>MASQPNSSAKKKEEKGKNIQVVVRCRPFNLAERKASAHSIVECDPVRKEVSVRTGGLADKSSRKTYTFDMVFGASTKQIDVYRSVVCPILDEVIMGYNCTIFAYGQTGTGKTFTMEGERSPNEEYTWEEDPLDGIIPRTLHQIFEKLTDNGTEFSVKVSLLEIYNEELFDLLNPSSDVSERLQMFDDPRNKRGVIIKGLEEITVHNKDEVYQILEKGAAKRTTAATLMNAYSSRSHSVFSVTIHMKETTIDGEELVKIGKLNLVDLAGSENIGRSGAVDKRAREAGNINQSLLTLGRVITALVERTPHVPYRESKLTRILQDSLGGRTRTSIIATISPASLNLEETLSTLEYAHRAKNILNKPEV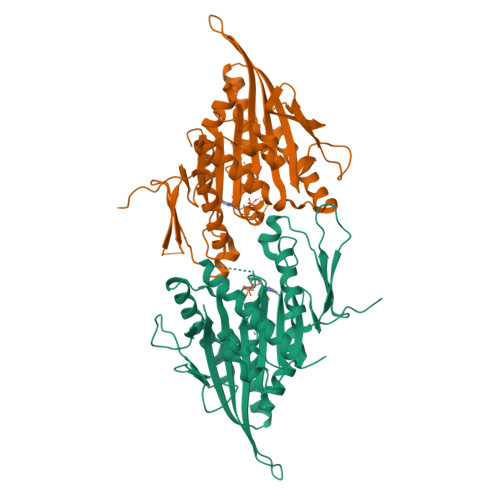NQK[2x]3-{2-[5-(difluoromethyl)-2H-thieno[3,2-c]pyrazol-3-yl]-1H-indol-6-yl}pentan-3-ol | 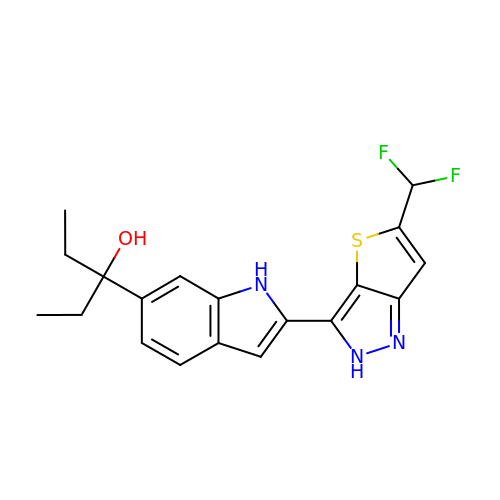C19 H19 F2 N3 O S | CQZZZUNOWZUNNG-UHFFFAOYSA-N> HHHHHHFNLPPGNYKKPVLLKSTETGQYLRINPDGTVDGTRDRSDTHIQFQISPEGNGEVLLKSTETGQYLRINPDGTVDGTRDRSDTHIQFQISPEGNGEV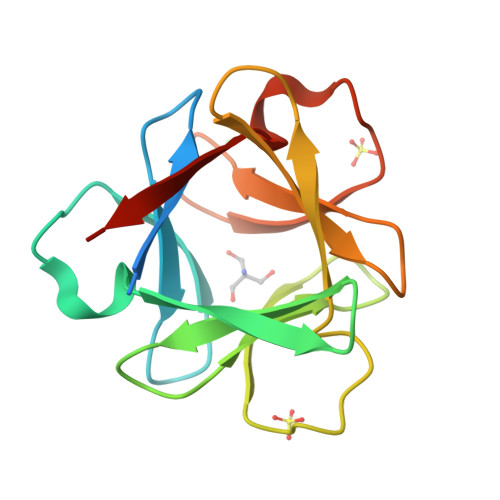LLKSTETGQYLRINPDGTVDGTRDRSDTHIQFQISPEGNG> MSLTDAKIRTLKPSDKPFKVSDSHGLYL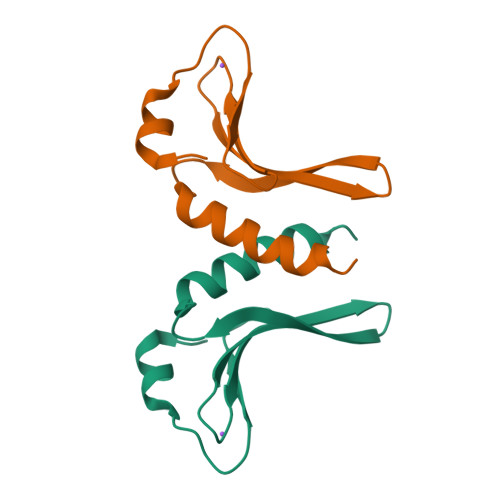LVKPGGSRHWYLKYRISGKESRIALGAYPAISLSDARQQREGIRKMLALNINLEHHHHHH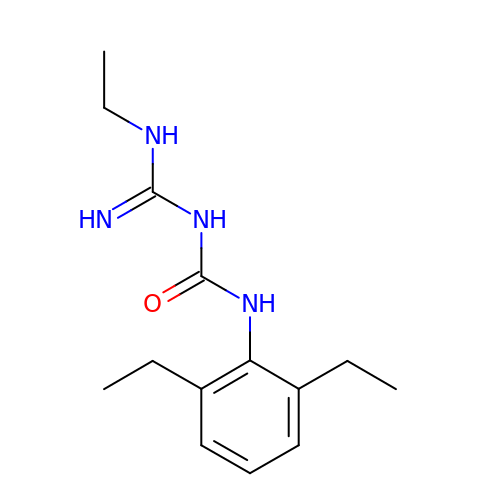N-(2,6-diethylphenyl)-N'-(N-ethylcarbamimidoyl)urea | C14 H22 N4 O | VHGRQUGTHVVVTE-UHFFFAOYSA-N>[3x]GPSPVGQQY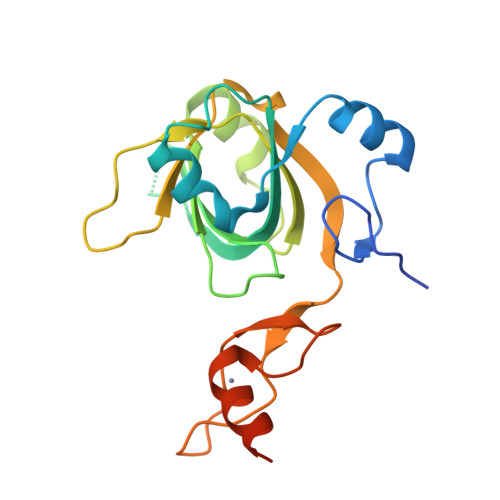HVEKFSGLRIRKPRVSSSEMERKMNGRKLIRLAQLQNKIATEKLEEEDWVTFGVIVKKITPQSSNNGKTFSIWRLNDLKDLDKYISLFLFGDVHKEHWKTDQGTVIGLLNANPMKPKEGTDEVCLSVDNPQKVLLMGDAVDLGTCKARKKNGDPCTQMVNLNDCEYCQYHVQAQYKKVSSKRADLQSSYSG> MDKYLDQFVKAPPAIKFGGLAFVVGALTAANFFMVIQPTEEEIGWAVAERRKLDLELADKSEIAQNLNERRREMDVLEQKLSEALTEL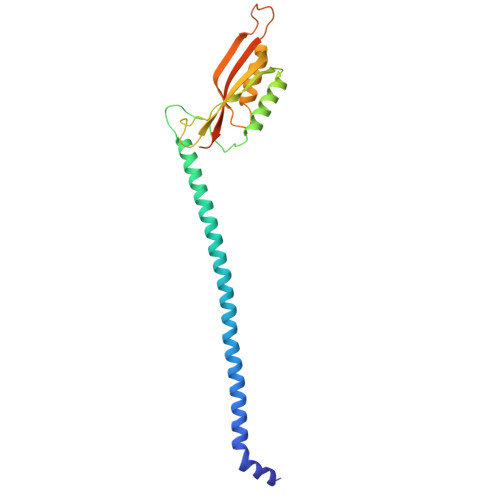PEQRDIEELLAQINDIGKKSGLELSSVTPGKESVGGGEFFARIPIKMTVSGNYHEIALFLQEMANMRRIVNVNNIKFDSAKLKNEKVVLQSEFQATTFRFVEQKAAASTAGNSNSKK>MVKLILVRAAESEWNPVGRYQGLLDPDLSERGKKQAKLLAQELSREHLDVIYSSPLKRTYLTALEIAEAKNLEVIKEDRIIEIDHGMWSGMLVEEVMEKYPEDFRRWVEEPHKVEFQGGESLASVYNRVKGFLEEVRKRHWNQTVVVVSHTVPMRAMYCALLGVDLSKFWSFGCDNASYSVIHM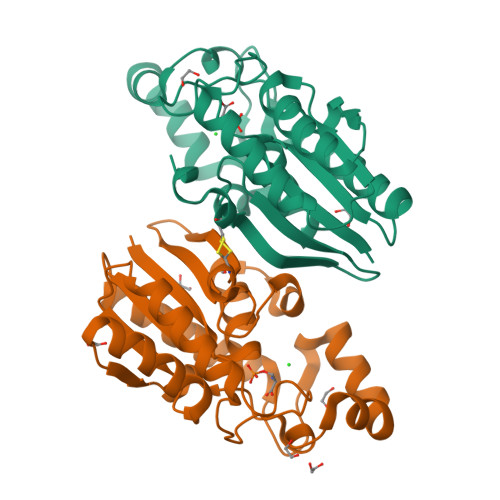EERRNVILKLNITCHLGEFYVEAHKAI[2x]>GGGGAUCUGUCACCCCAUUGAUCGCCUUCGGGCUGAUCUGG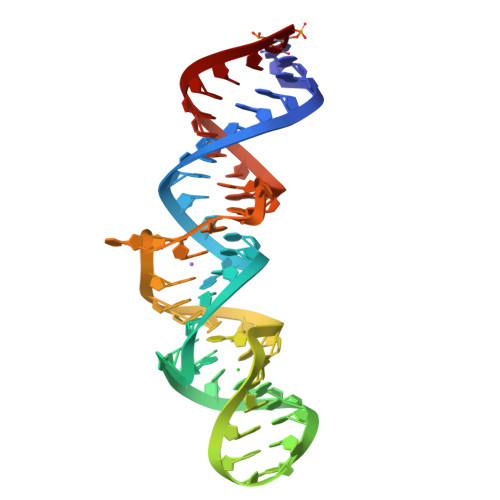CUGGCUAGGCGGGUCCC[2x]> MTQEVDQQILLQQLKSDYRQILLSYFTTDKALKEKIDKFINAVFCANIPVPEIIEIHMELIDEFS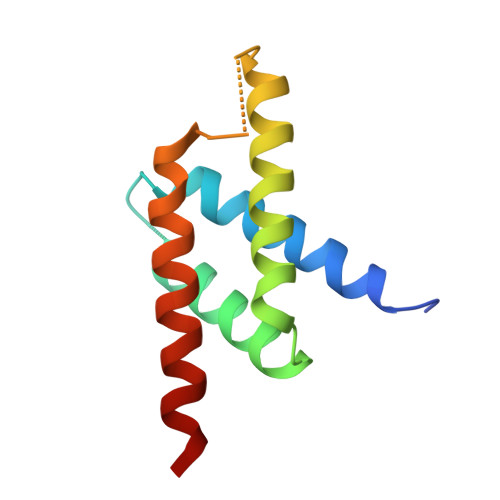KQLRLEGRGDETLMDYRLTLIDILAHLCEAYRGAIFK> MDQSSHHHHHHALDLGSAEAKAWIGVENPHRADVLTE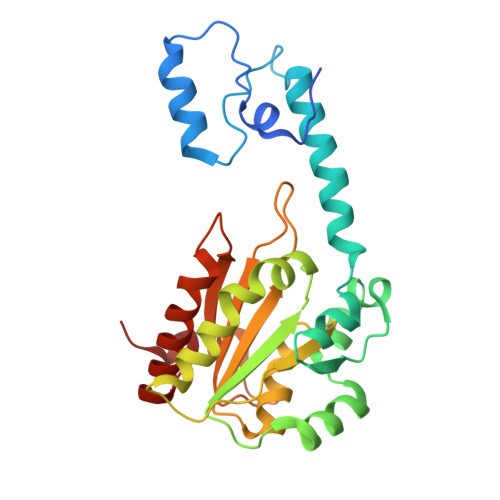LRRSTVARVCTGRAGPRPRTQALLRFLADHSRSKDTVLKEVPEEWVKAQGLLEVRSEISDKNLYLTRPDMGRRLCAEAVEALKAQCVANPDVQVVISDGLSTDAITVNYEEILPPLMAGLKQAGLKVGTPFFVRYGRVKIEDQIGEILGAKVVILLVGERPGLGQSESLSCYAVYSPRMATTVEADRTCISNIHQGGTPPVEAAAVIVDLAKRMLEQKASGINMTR> 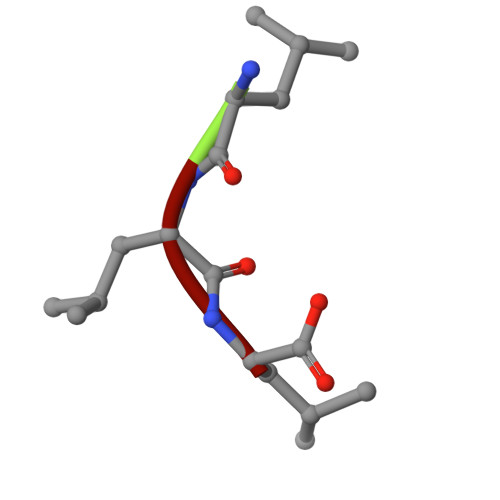LLL>[2x]XEVEALEKKVEAL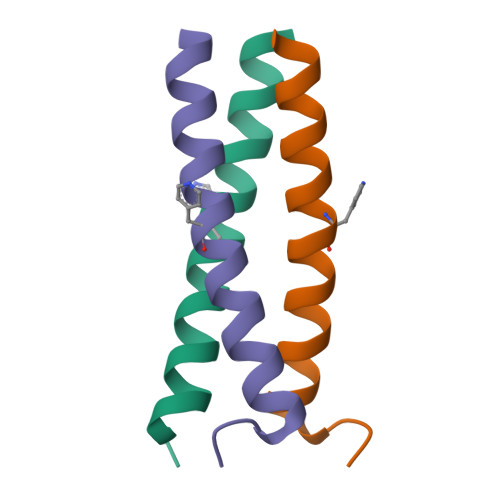EXKVQKLEKKVEALEHGWDGR SINAPINATE | C11 H12 O5 | 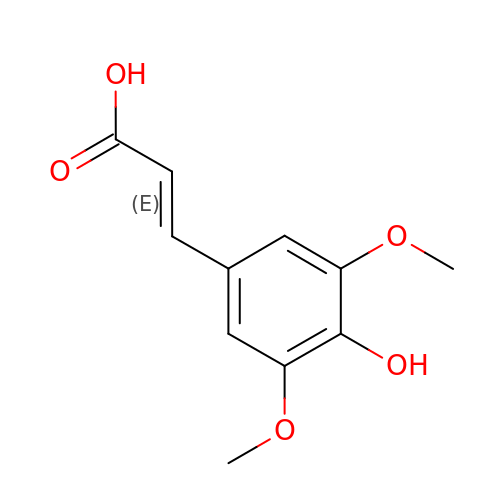PCMORTLOPMLEFB-ONEGZZNKSA-N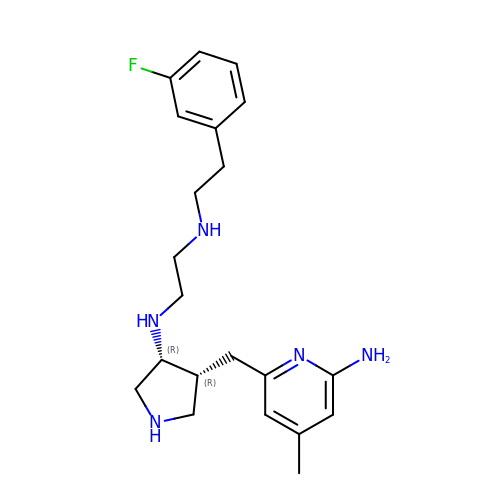N-{(3R,4R)-4-[(6-amino-4-methylpyridin-2-yl)methyl]pyrrolidin-3-yl}-N'-[2-(3-fluorophenyl)ethyl]ethane-1,2-diamine | C21 H30 F N5 | PUOKPLCASUFBAN-XLIONFOSSA-N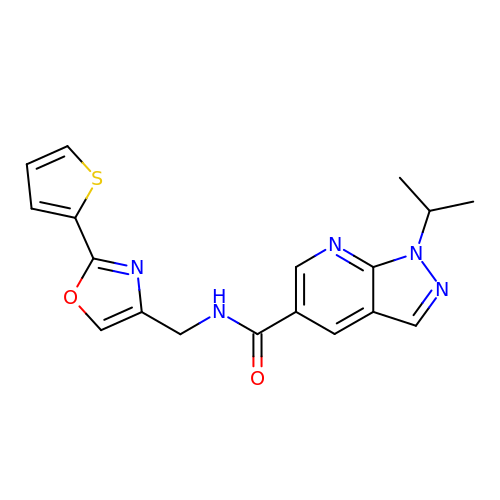1-(propan-2-yl)-N-{[2-(thiophen-2-yl)-1,3-oxazol-4-yl]methyl}-1H-pyrazolo[3,4-b]pyridine-5-carboxamide | C18 H17 N5 O2 S | OISFTLSEOJZOQD-UHFFFAOYSA-N2-(3,4-dihydroxyphenyl)-5-hydroxy-4H-1-benzopyran-4-one 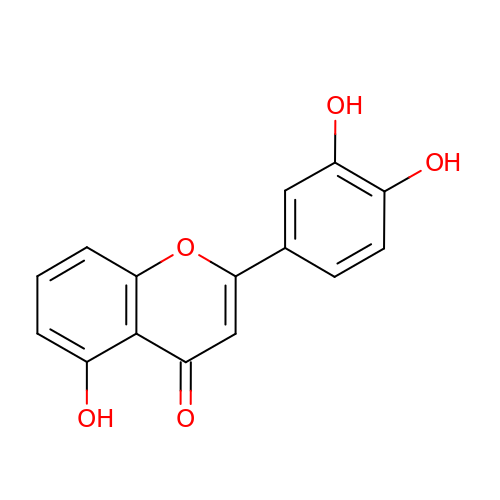| C15 H10 O5 | KXPQYWKYYDYOCQ-UHFFFAOYSA-N> MKLPVREFDAVVIGAGGAGMRAALQISQSGQTCALLSKVFPTRSHTVSAQGGITVALGNTHEDNWEWHMYDTVKGSDYIGDQDAIEYMCKTGPEAILELEHMGLPFSRLDDGRIYQRPFGGQSKNFGGEQAARTAAAADRTGHALLHTLYQQNLKNHTTIF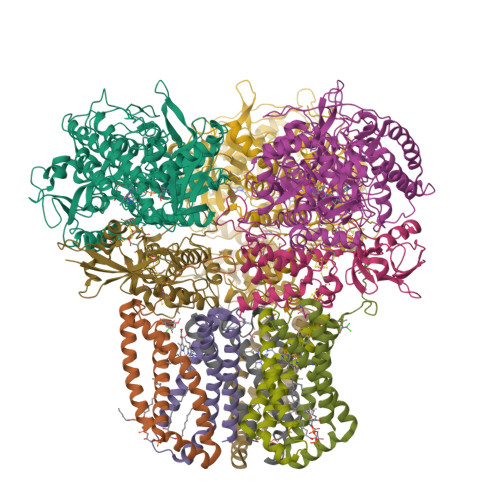SEWYALDLVKNQDGAVVGCTALCIETGEVVYFKARATVLATGGAGRIYQSTTNAHINTGDGVGMAIRAGVPVQDMEMWQFHPTGIAGAGVLVTEGCRGEGGYLLNKHGERFMERYAPNAKDLAGRDVVARSIMIEIREGRGCDGPWGPHAKLKLDHLGKEVLESRLPGILELSRTFAHVDPVKEPIPVIPTCHYMMGGIPTKVTGQALTVNEKGEDVVVPGLFAVGEIACVSVHGANRLGGNSLLDLVVFGRAAGLHLQESIAEQGALRDASESDVEASLDRLNRWNNNRNGEDPVAIRKALQECMQHNFSVFREGDAMAKGLEQLKVIRERLKNARLDDTSSEFNTQRVECLELDNLMETAYATAVSANFRTESRGAHSRFDFPDRDDENWLCHSLYLPESESMTRRSVNMEPKLRPAFPPKIRTY;> MRLEFSIYRYNPDVDDAPRMQDYTLEADEGRDMMLLDALIQLKEKDPSLSFRRSCREGVCGSDGLNMNGKNGLACITPISALNQPGKKIVIRPLPGLPVIRDLVVDMGQFYAQYEKIKPYLLNNGQNPPAREHLQMPEQREKLDGLYECILCACCSTSCPSFWWNPDKFIGPAGLLAAYRFLIDSRDTETDSRLDGLSDAFSVFRCHSIMNCVSVCPKGLNPTRAIGHIKSMLLQRNA;> MIRNVKKQRPVNLDLQTIRFPITAIASILHRVSGVITFVAVGILLWLLGTSLSSPEGFEQASAIMGSFFVKFIMWGILTALAYHVVVGIRHMMMDFGYLEETFEAGKRSAKISFVITVVLSLLAGVLVW;> MVSNASALGRNGVHDFILVRATAIVLTLYIIYMVGFFATSGELTYEVWIGFFASAFTKVFTLLALFSILIHAWIGMWQVLTDYVKPLALRLMLQLVIVVALVVYVIYGFVVVWGV> MEEPEEPADSGQSLVPVYIYSPEYVSMCDSLAKIPKRASMVHSLIEAYALHKQMRIVKPKVASMEEMA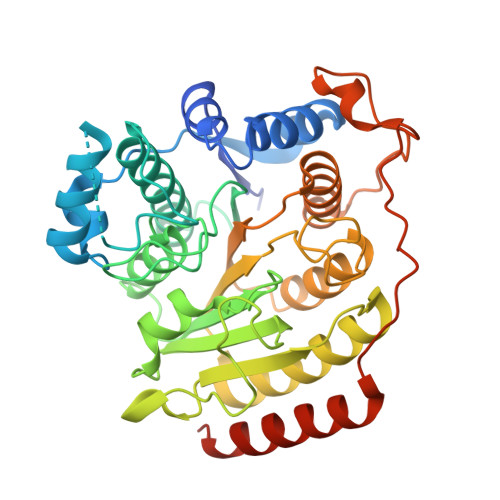TFHTDAYLQHLQKVSQEGDDDHPDSIEYGLGYDCPATEGIFDYAAAIGGATITAAQCLIDGMCKVAINWSGGWHHAKKDEASGFCYLNDAVLGILRLRRKFERILYVDLDLHHGDGVEDAFSFTSKVMTVSLHKFSPGFFPGTGDVSDVGLGKGRYYSVNVPIQDGIQDEKYYQICESVLKEVYQAFNPKAVVLQLGADTIAGDPMCSFNMTPVGIGKCLKYILQWQLATLILGGGGYNLANTARCWTYLTGVILGKTLSSEIPDHEFFTAYGPDYVLEITPSCRPDRNEPHRIQQILNYIKGNLKHVVIEGRGSHHHHHH>DALKVNRAPVGVEPQEVHKWLQSFNWDFKENRTKYPTKYHMANETKEQFKVIAKEYARMEAAKDERQFGTLLDGLTRLGAGNKVHPRWGETMKVISNFLEVGEYNAIAASAMLWDSATAAEQKNGYLAQVLDEIRHTHQCAFINHYYSKHYHDPAGHNDARRTRAIGPLWKGMKRVFADGFISGDAVECSVNLQLVGEACFTNPLIVAVTEWASANGDEITPTVFLSVETDELRHMANGYQTVVSIANDPASAKFLNTDLNNAFWTQQKYFTPVLGYLFEYGSKFKVEPWVKTWNRWVYEDWGGIWIGRLGKYGVESPASLRDAKRDAYWAHHDLALAAYAMWPLGFARLALPDEEDQAWFEANYPGWADHYGKIFNEWKKLGYEDPKSGFIPYQWLLANGHDVYIDRVSQVPFIPSLAKGTGSLRVHEFNGKKHSLTDDWGERQWLIEPERYECHNVFEQYEGRELSEVIAEGHGVRSDGKTLIAQPHTRGDNLWTLEDIKRAGCVFPDPLAKF[2x];>[2x]PQSSQVTKRGLTDPERAAIIAAAVPDHALDTQRKYHYFIQPRWKRLSEYEQLSCYAQPNPDWIAGGLDWGDWTQKFHGGRPSWGNESTELRTTDWYRHRDPARRWHHPYVKDKSEEARYTQRFLAAYSSEGSIRTIDPYWRDEILNKYFGALLYSEYGLFNAHSSVGRDCLSDTIRQTAVFAALDKVDNAQMIQMERLFIAKLVPGFDASTDVPKKIWTTDPIYSGARATVQEIWQGVQDWNEILWAGHAVYDATFGQFARREFFQRLATVYGDTLTPFFTAQSQTYFQTTRGAIDDLFVYCLANDSEFGAHNRTFLNAWTEHYLASSVAALKDFVGLYAKVEKVAGATDRAGVSEALQRVFGDWKIDYADKIGFRVDVDQKVDAVLAGYKN;>AKREPIHDNSIRTEWEAKIAKLTSVDQATKFIQDFRLAYTS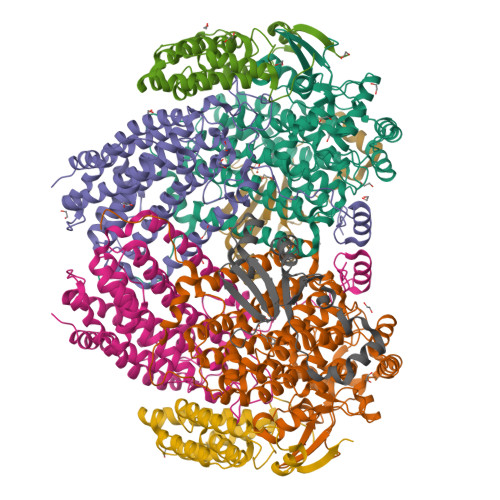PFRKSYDIDVDYQYIERKIEEKLSVLKTEKLPVADLITKATTGEDAAAVEATWIAKIKAAKSKYEAERIHIEFRQLYKPPVLPVNVFLRTDAALGTVLMEIRNTDYYGTPLEGLRKERGVKVLHLQA[2x];>SAHNAYNAGIMQKTGKAFADEFFAEENQVVHESNAVVLVLMKSDEIDAIIEDIVLKGGKAKNPSIVVEDKAGFWWIKADGAIEIDAAEAGELLGKPFSVYDLLINVASAVGRAYTLGTKFTITSELMGLDR[2x]> GAMGGSEFPKSRLPTLADNEIEYEKQIGKGGFGLVHKGRLVKDKSVVAIKSLILGDSEGETEMIEKFQEFQREVFIMSNLNHPNIVKLYGL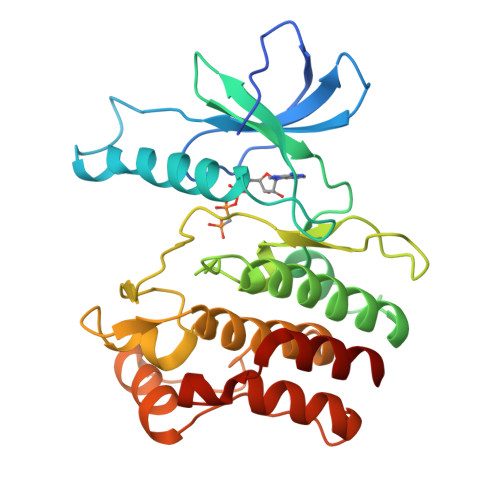MHNPPRMVMEFVPCGDLYHRLLDKAHPIKWSVKLRLMLDIALGIEYMQNQNPPIVHRDLRSPNIFLQSLDENAPVCAKVADFGTSQQSVHSVSGLLGNFQWMAPETIGAEEESYTEKADTYSFAMILYTILTGEGPFDEYSYGKIKFINMIREEGLRPTIPEDCPPRLRNVIELCWSGDPKKRPHFSYIVKELSEL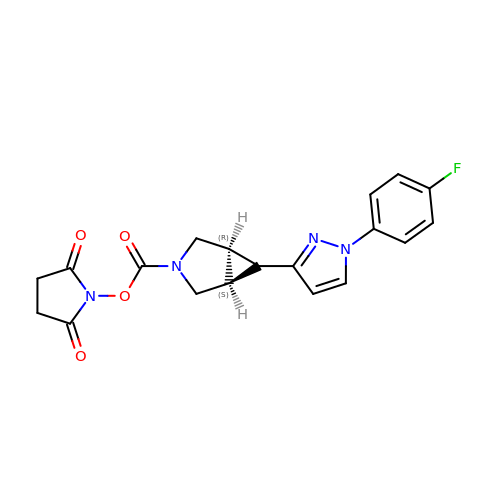1-({(1R,5S,6r)-6-[1-(4-fluorophenyl)-1H-pyrazol-3-yl]-3-azabicyclo[3.1.0]hexane-3-carbonyl}oxy)pyrrolidine-2,5-dione | C19 H17 F N4 O4 | FNIBKVOGYHDUDM-UOIKSKOESA-N>[2x]MGDLMIHLQAPDLGSLNSGSLVYFRKIPVGKVYDYAINPNKQGVVIDVLIERRFTDLVK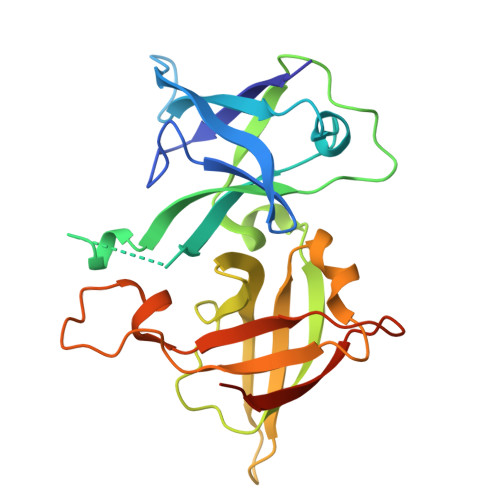KGSRFWNVSGVDANVSISGAKVKLESLAALVNGAIAFDSPEESKPAEAEDTFGLYEDLAHSQRGVIIKLELPSGAGLTADSTPLMYQGLEVGQLTKLDLNPGGKVTGEMTVDPSVVTLLRENTRIELRNPKLSLSDANLSALLTGKTFELVPGDGEPRKEFVVVPGEGETHHHHHH> GPAMSPESKNAVQMQSEKSASDSGEVATEKAPAKQDTKEKSGTETEKGKEDGTKGTKDSSADKETSAEASEKGTVVTETADDDLFTTYRLDLEDARSKEREELNAIVSSDDATAKEK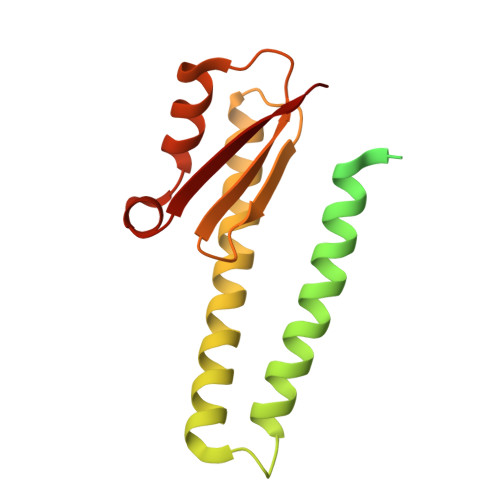SEAYDKMTALSEVEGTEKQLETLIKTQGYEDALVNAEGDKINITVKSDKHSKSKATAIIDLVAKEIKTMKDVAVTFEPSK> MERTELLKPRTLADLIRILHELFAGDEVNVEEVQAVLEAYESNPADWALYAKFDQYRYTRNLVDQGNGKFNLMILCWGEGHGSS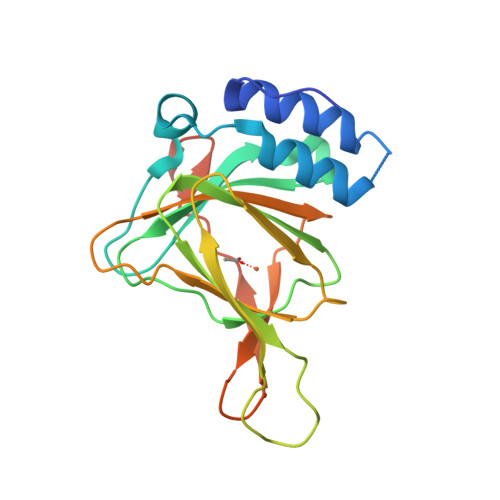IHDHTDSHEFLKLLQGNLKETLFDWPDKKSNEMIKKSERTLRENQCAYINDSIGLHRVENVSHTEPAVSLHLYSPPFDTCHAFDQRTGHKNKVTMTFHSKFGIRTPFTTSGSLENN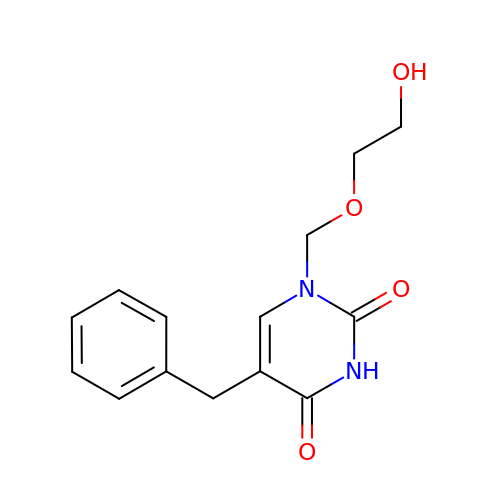1-((2-HYDROXYETHOXY)METHYL)-5-BENZYLPYRIMIDINE-2,4(1H,3H)-DIONE | C14 H16 N2 O4 | SPJAGILXQBHHSZ-UHFFFAOYSA-N> MDHAEENEILAATQRYVVERPVYSQELLEEELEKKDRVPKTLGDKLKKSFRCSPKKAKNLLLSFFPILEWLPKYNLKEWLLGDLIAGLTVGSLQIPQGIAFALLAGLPPIYGLYSSFFPPLIYAFFGTSRHISVGPFAVVSLLVGSVVERLVPDDIVLPGGVNATNGTEARDALRVQVAFTLTFLAGIIQLALGLLRLGFLVDFLSEPLISGFTTGAAIHILLSQLKYLLGLKIPRHSGPFSVIYSVISVFHNIPNTNIATLGVSLLSFVLLLVVKELNKRFKKKLPVPIPAELIVVILATLISYYFNLAEKYGVSIVGHIPKGLPPPSVPDLSLFPLVIGDAIAIAIVGLAVSISVGKTFAKKHGYQIDGNQELIALGLMNIVGSFFSCYPATGSFSRSAVNESAGGKTQVAGIVAALVVLLVLLFLGPL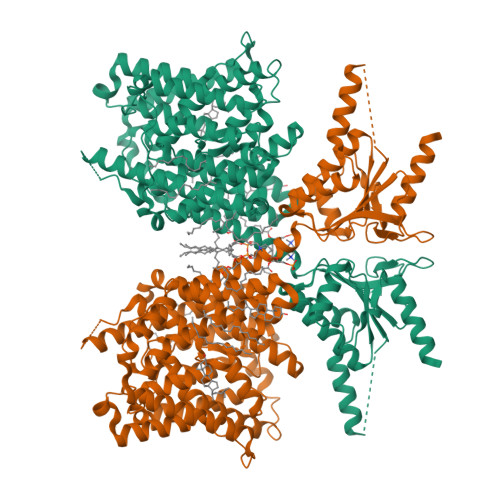FYYLPKAVLAAIIIVNLKGLLMQFKDAPKLWKVDKLDFLIWLVTFLGVVFLSVEIGLLVGVGFSLLTVLLRTQRPRTSVLGRIPGTDIYRDVKQYPEAEEVPGVKIFRIDSPIYFANSEYFKERLKRKTGVDPVKVLAARKKALKKIEKEIKKANLANKTVVKADAEVDGEDATKPEEEDGEVKYPPIVIQSDWPSELPRFVPPKVDFHTLILDFSAVSFVDTVGVKTLKEIVKEYREIGVQVYLAGCNASVVEKLERGGFFDDGITKEHLFLSVHDAVLFAQARKALAEQEASAPPSQEDLEPNATPATPEAGTENLYFQG>GG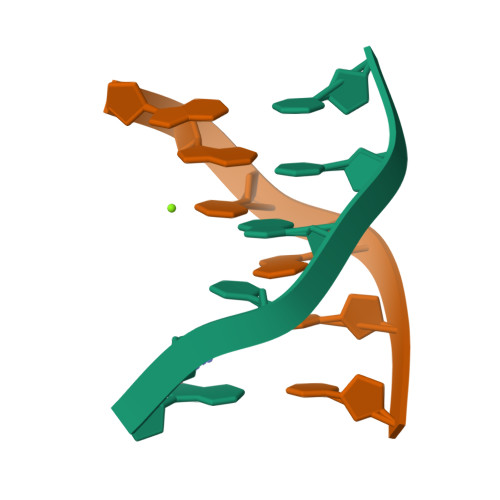CGCC[2x]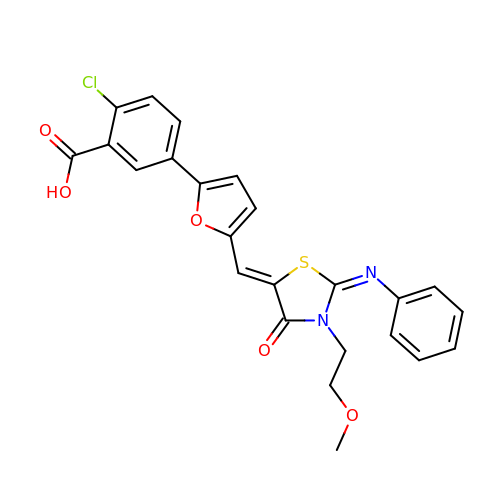2-CHLORO-5-(5-{(E)-[(2Z)-3-(2-METHOXYETHYL)-4-OXO-2-(PHENYLIMINO)-1,3-THIAZOLIDIN-5-YLIDENE]METHYL}-2-FURYL)BENZOIC ACID | C24 H19 Cl N2 O5 S | BLYOIVXXTIAFFL-QPVYCHHJSA-N2-DEAZO-6-THIOPHOSPHATE GUANOSINE-5'-MONOPHOSPHATE | C10 H15 N4 O10 P2 S | 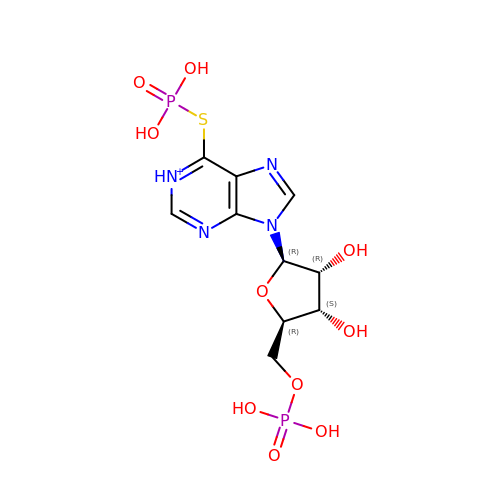NYBPOGVUIOPXHI-KQYNXXCUSA-O> GSTAEKDKLPATQKAKEMQNVPYTIAVDGIMAFNQSYLNLPKD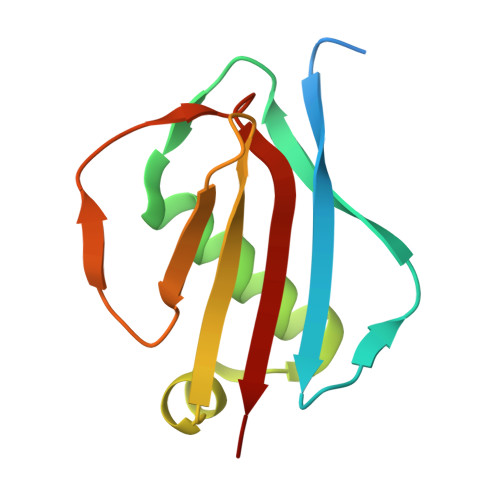SQLSYLDLGNKVKALLYDERGVTPEKIRNAKSAVYTITWKDGSKKEVDLKKDSYTANLFDSNSIKQIDINVKTK> MHHHHHHVPAILVNDEQWLGESAVARMTTRAQGLEELYKLWGYRATRIDTMCEQPSTSIFQCQVRQLNWQELQQTPHPLLLTLQHEGQRAYVVLLEVDPERVVLLTGEQRLTFTVSQLMSLWRGEVTDLWPMPLRETLRLGMHGEAIEVLDQLLAKALNDEPLKTTQFNAELMQRVEWFQRWQAMTEDGIAGQRTLARLQHMVSLSEPWRALTQAEKQGEEQVMRYPEFPSLAPLLRTYPLAETGDVINVADQTS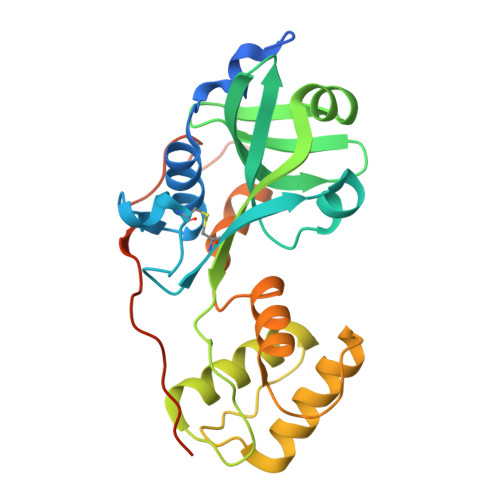PTL>GSHMGNNICIDDNINTLWTGVNPTEANCQMMDSSESNDCKLILTLVKTGALVTAFVYVIGVSNNFNMLTTYRNINFTAELFFDSAGNLLTSLSSLKTPLNHKSGQNMATGAITNAKSFMPSTTAYPFNNNSREKENYIYGTCHYTASDHTAFPIDISVMLNQRAIRADTSYCIRITWSWNTGDAPEGQTSATTLVTSPFTF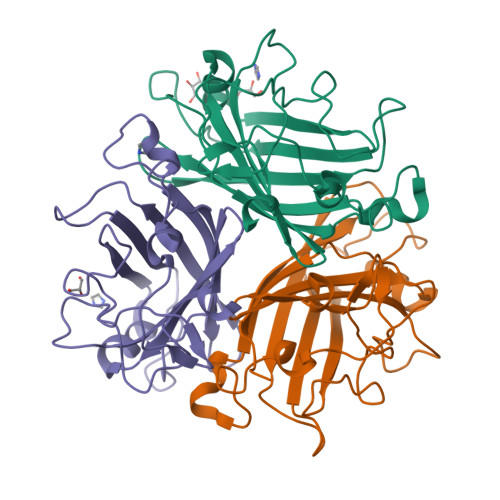YYIREDD[9x]>MRKLAHNFYKPLAIGAPEPIRELPVRPERVVHFFPPHVEKIRARIPEVAKQVDVLCGNLEDAIPMDAKEAARNGFIEVVKATDFGDTALWVRVNALNSPWVLDDIAEIVAAVGNKLDVIMIPKVEGPWDIHFVDQYLALLEARHQIKKPILIHALLETAQGMVNLEEIAGASPRMHGFSLGPADLAASRGMKTTRVGGGHPFYGVLADPQEGQAERPFYQQDLWHYTIARMVDVAVAHGLRAFYGPFGDIKDEAACEAQFRNAFLLGCTGAWSLAPNQIPIAKRVFSPDVNEVLFAKRILEAMPDGSGVAMIDGKMQDDATWKQAKVIVDLARMIAKKDPDLAQAYGL[6x]

Malyl-CoA lyase (MCL) is a promiscuous carbon-carbon bond lyase that catalyzes the reversible cleavage of structurally related Coenzyme A (CoA) thioesters. Malyl-CoA lyases are promiscuous enzymes that accept a variety of substrates and can catalyze the reversible aldol condensation of CoA thioesters like acetyl-CoA or propionyl-CoA with 2-oxoacids like glyoxylate or pyruvate. The two MCLs share the common fold of a central TIM-barrel with small elaborations, as well as an additional C-terminal domain. In both cases the oligomeric state constitutes a dimer of trimers.

Subsequently it was discovered that in C. aurantiacus an MCL (MCLC) catalyzes three different steps in the 3-hydroxypropionate bi-cycle for autotrophic CO2 fixation. In the absence of substrates recombinant MCLC crystallized in the orthorhombic space group P 2 21 21 with one hexamer per asymmetric unit (AU). The crystals diffracted to a resolution of 2.5 Å and the structure was solved using the molecular replacement method. Only 4 to 6 residues were not built in a loop region (residues 210 – 215) of each chain due to the lack of sufficient electron density. As with other members of the CitE-like superfamily and malate synthases, the core of the MCLC monomer constitutes a β8/α8 TIM-barrel. In addition to the central TIM-barrel there is a C-terminal domain (starting at Phe287) that comprises three α-helices of which two are connected by a β-hairpin (residues 310–317). This C-terminal domain extends to the neighboring subunit. In both MCLC structures (with and without bound substrates) additional electron density was observed at the 3-fold rotation axis in each trimer and was modeled as Tris molecules. These form hydrogen bonds with the side chain amide oxygens of Gln221 in each subunit of the trimer, as well as with backbone oxygen atoms of Asp222. The Tris molecules are buried within the protein and do not appear to be solvent accessible, which may indicate that the additional insertion domain (residues 182–220) found after the sixth β-strand of the TIM-barrel is able to undergo a conformational change.>MVEIFNEIMQRVKEAETIIIHRHVRPDPDAYGSQLGLKLYLERKFPEKNIYATGEAEPSLSFIGDLDEIDDSVYSDALVIVCDTANAPRIDDQRYLNGQSLIKIDHHPATDQYGDVNFVNTEASSTSEIIFDFISHFNDLSIIDEHVARVLYLGIVGDTGRFLFSNTSPHTMEVASQLLAYPFNHNAELNKMSEKDPKLMPFQGYVLQNFELSDSHEYCQIKITNDVLKQFDIQPNEASQFVNTVADISGLKIWMFGVD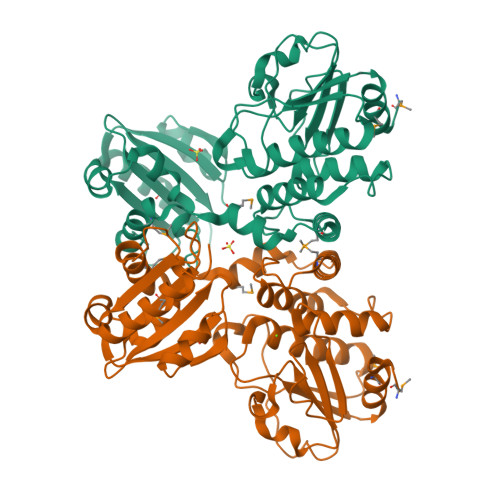EGDQIRCRIRSKGITINDVANQFGGGGHPNASGVSVYSWDEFEELAQALRQKLLEHHHHHH[2x]>SATYQFDPSHTYPSFEADHFGGLSVWRGKFDKSSGTVTLDRAAKTGTVDVTTDIASIHTGSAKLDEHLQTAEFFDAAKFPQANYKGTIKFDGDKPVSVVGNLTLHGVTKPLTLKIDSFKCMPHPMLKREV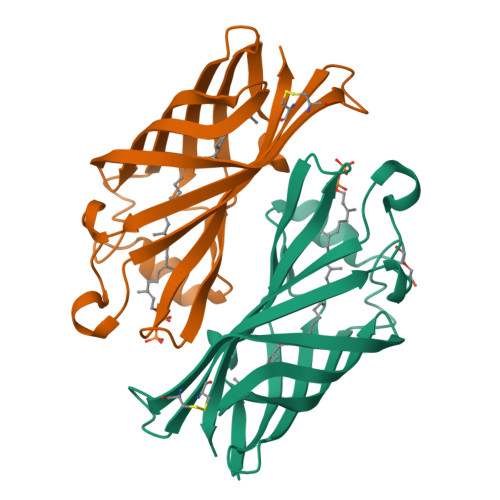CGVDAVGEFSRDDFGLDYGKQYGFKMKTKLLITAEAVKQ[4x]>FTLIELMIVVAIIGILAAIAIPQYQNYVARSEGASALATINPLKTTVEESLSRGI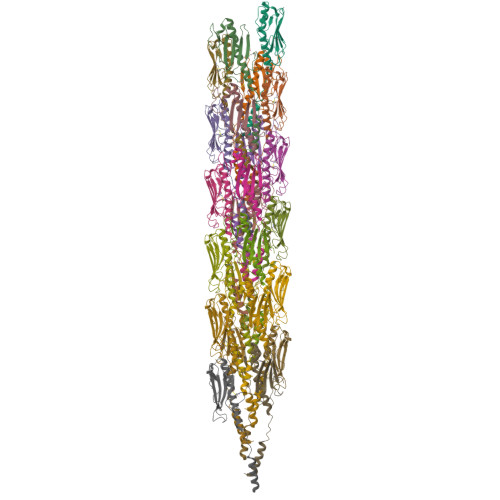AGSKIKIGTTASTATETYVGVEPDANKLGVIAVAIEDSGAGDITFTFQTGTSSPKNATKVITLNRTADGVWACKSTQDPMFTPKGCDN[23x]>[2x]MRSRRVDVMD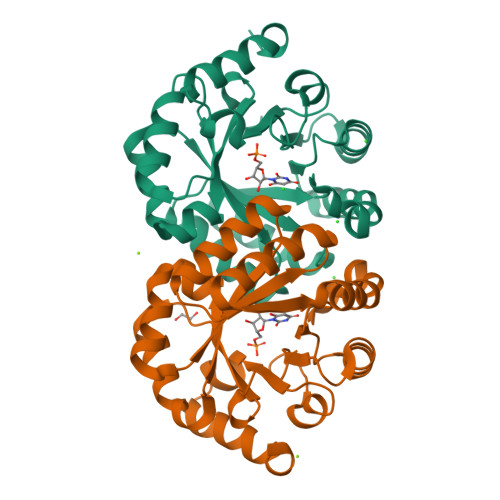VMNRLILAMDLMNRDDALRVTGEVREYIDTVKIGYPLVLSEGMDIIAEFRKRFGCRIIADFKVADIPETNEKICRATFKAGADAIIVHGFPGADSVRACLNVAEEMGREVFLLTEMSNPGAEMFIQGAADEIARMGVDLGVKNYVGPSTRPERLSRLREIIGQDSFLISPGVGAQGGDPGETLRFADAIIVGRSIYLADNPAAAAAGIIESIKDLLNP> SNIPYTQLDMAVVQNRPAGSLRRFVVLVVGETTRAANWGLNGYSRQTTPLLAARGDEIVNFPQVRSCGTSTAHSLPCMFSTFDRTDYDEIKAEHQDNLLDIVQRAGVEVTWLENDSGCKGVCGKVPNTDVTSLNLPEYCRNGECLDNILLTKFDEVL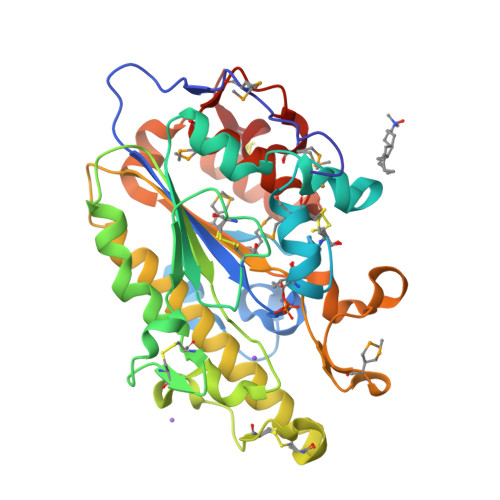NKNDKDAVLILHTIGSHGPTYYERYTEAERKFTPTCDTNEINKCTRATLVNTYDNTVLYVDQFIDKVIRKLENRDDLESVVHYVSDHGESLGENGMYLHAAPYAIAPSGQTHIPMVMWFSKAFRQHGGIDFQCLKQKAAENEYSHDHYFSTVLGLMDISNSQTYRKEMDILAACRRPR>[4x]MQFPQLDPATLAAFSAAFRGELIWPSDADYDEARRIWNGTIDRRPALIARCTSTPDVVAAVSFARKSGLLVAVRGGGHSMAGHSVCDGGIVIDLSLMNSIKVSRRLRRARAQGGCL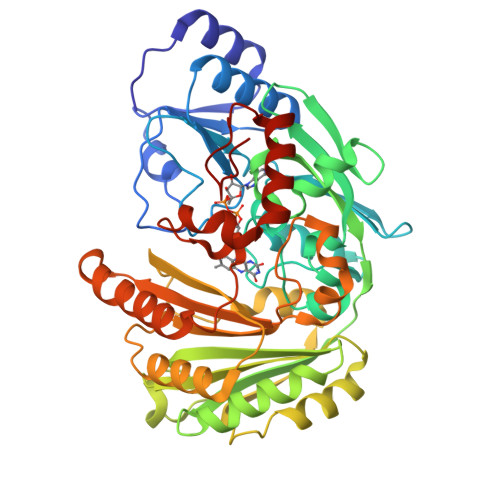LGAFDTATQAHMLATPAGTVSHTGLGGLVLGGGFGWLSRKYGLSIDNLTSVEIVTADGGVLTASDTENPDLFWAVRGGGGNFGVVTAFEFDLHRVGPVRFASTYYSLDEGPQVIRAWRDHMATAPDELTWALYLRLAPPLPELPADMHGKPVICAMSCWIGDPHEGERQLESILHAGKPHGLTKATLPYRALQAYSFPGAVVPDRIYTKSGYLNELSDEATDTVLEHAADIASPFTQLELLYLGGAVARVPDDATAYPNRQSPFVTNLAAAWMDPTEDARHTAWAREGYRALAGHLSGGYVNFMNPGEADRTREAYGAAKFERLQGVKAKYDPTNLFRLNQNIPPSSP> MGSDKIHHHHHHMDLELKELQSKMKEMYFEKDSQRGIYATFTWLVEEVGELAEALLSNNLDSIQEELADVIAWTVSIANLEGIDIEEALKKKY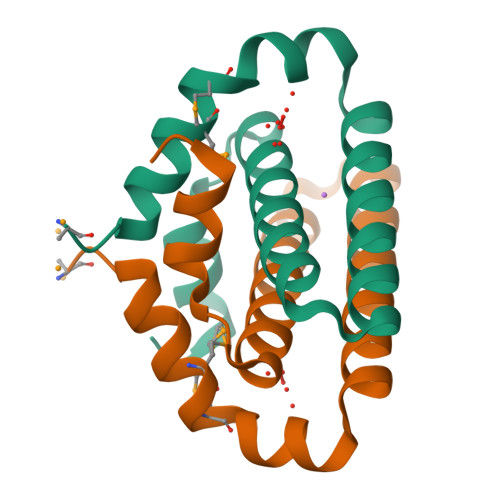KL>[2x]MIDYTAAGFTLLQGAHLYAPEDRGICDVLVANGKIIAVASNIPSDIVPNCTVVDLSGQILCPGFIDQHVHLIGGGGEAGPTTRTPEVALSRLT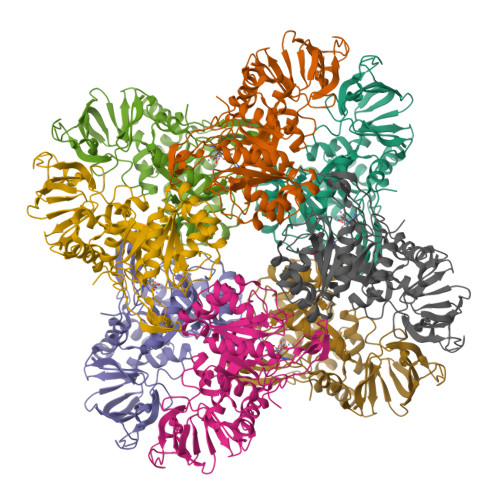EAGVTSVVGLLGTDSISRHPESLLAKTRALNEEGISAWMLTGAYHVPSRTITGSVEKDVAIIDRVIGVKCAISDHRSAAPDVYHLANMAAESRVGGLLGGKPGVTVFHMGDSKKALQPIYDLLENCDVPISKLLPTHVNRNVPLFEQALEFARKGGTIDITSSIDEPVAPAEGIARAVQAGIPLARVTLSSNGNGSQPFFDDEGNLTHIGVAGFETLLETVQVLVKDYDFSISDALRPLTSSVAGFLNLTGKGEILPGNDADLLVMTPELRIEQVYARGKLMVKDGKACVKGTFETA> MFYALYFEIHHLVASAALGFARVAPIFFFLPFLNSGVLSGAPRNAIIILVAL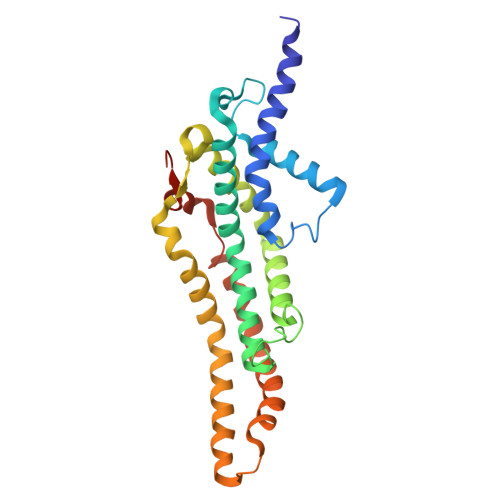GVWPHALNEAPPFLSVAMIPLVLQEAAVGVMLGCLLSWPFWVMHALGCIIDNQRGATLSSSIDPANGIDTSEMANFLNMFAAVVYLQNGGLVTMVDVLNKSYQLCDPMNECTPSLPPLLTFINQVAQNALVLASPVVLVLLLSEVFLGLLSRFAPQMNAFAISLTVKSGIAVLIMLLYFSPVLPDNVLRLSFQATGLSSWFYERGATHVLE7-{[3-({[3-(6-aminopyridin-2-yl)propyl]amino}methyl)phenoxy]methyl}quinolin-2-amine | 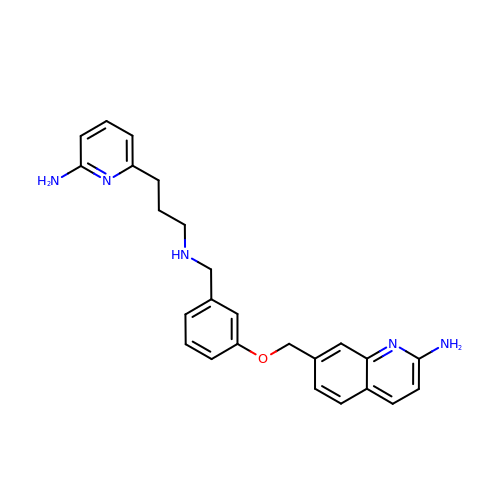C25 H27 N5 O | YWEAUSOYABUBID-UHFFFAOYSA-N>[4x]MRIPLVGKDSIESKDIGFTLIHEHLRVFSEAVRQQWPHLYNEDEEFRNAVNEVKRAMQFGVKTIVDP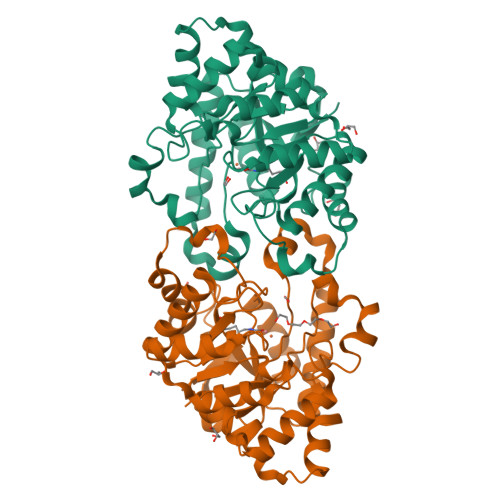TVMGLGRDIRFMEKVVKATGINLVAGTGIYIYIDLPFYFLNRSIDEIADLFIHDIKEGIQGTLNKAGFVKIAADEPGITKDVEKVIRAAAIANKETKVPIITHSNAHNNTGLEQQRILTEEGVDPGKILIGHLGDTDNIDYIKKIADKGSFIGLDRYGLDLFLPVDKRNETTLRLIKDGYSDKIMISHDYCCTIDIGTAKPEYKPKLAPRWSITLIFEDTIPFLKRNGVNEEVIATIFKENPKKFFS>[2x]SEPSTTNKPIVLSTWNFGLHANVEAWKVLSKGGKALDAVEKGVRLVEDDPTERSVGYGGRPDRDGRVTLDACIMDENYNIGSVACMEHIKNPIS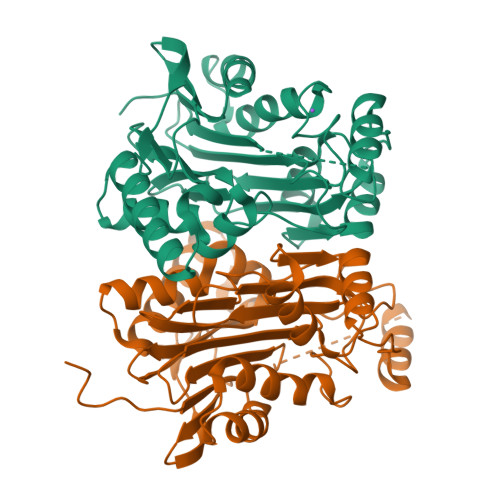VARAVMEKTPHVMLVGDGALEFALSQGFKKENLLTAESEKEWKEWLKTSQYKPIVNIENHDCIGMIALDAQGNLSGACTTSGMAYKMHGRVGDSPIIGAGLFVDNEIGAATATGHGEEVIRTVGTHLVVELMNQGRTPQQACKEAVERIVKIVNRRGKNLKDIQVGFIALNKKGEYGAYCIQDGFNFAVHDQKGNRLETPGFALK> ALTQSVGGDSSADRLFPPQWICCDIRYLDVSILGKFAVVMADPPWDIHMELPYGTLTDDEMRRLNIPVLQDDGFLFLWVTGRAMELG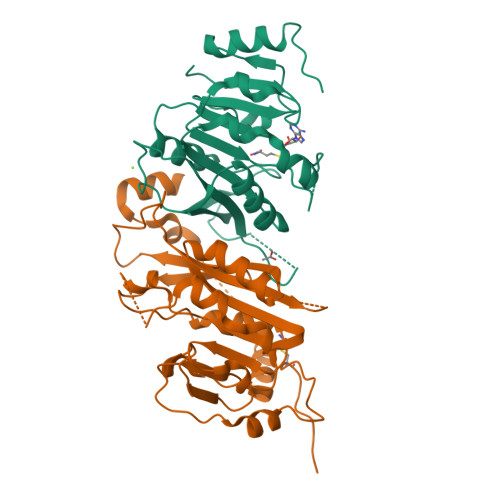RECLNLWGYERVDEIIWVKTNQLQRIIRTGRTGHWLNHGKEHCLVGVKGNPQGFNQGLDCDVIVAEVRSTSHKPDEIYGMIERLSPGTRKIELFGRPHNVQPNWITLGNQLDGIHLLDPDVVARFKQRYPDGIISKPKNL;> LKGTQSLNPHNDYCQHFVDTGHRPQNFIRDVGLADRFEEYPKLRELIRLKDELIAKSNTPPMYLQADIEAFDIRELTPKFDVILLEPPLEEYYRETGITANEKCWTWDDIMKLEIDEIAAPRSFIFLWCGSGEGLDLGRVCLRKWGYRRCEDICWIKTNKNNPGKTKTLDPKAVFQRTKEHCLMGIKGTVKRSTDGDFIHANVDIDLIITEEPEIGNIEKPVEIFHIIEHFCLGRRRLHLFGRDSTIRPGWLTVGPTLTNSNYNAETYASYFSAPNSYLTGCTEEIERL>[4x]IEKKIVLRNGTEAFDSWEKPPLPVYTQFYFFNVTNPEEILRGETPRVEEVGPYTYRELRNKANIQFGDNGTTISAVSNKAYVFERDQSVGDPKIDLIRTLNIPVLTVIEWSQVHFLREIIEAMLKAYQQKLFVTHTVDELLWGYKDEILSLIHVFRPDISPYFGLFYEKNGTNDGDYVFLTGEDS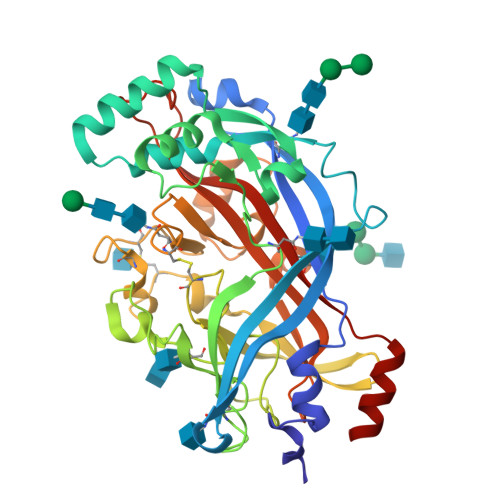YLNFTKIVEWNGKTSLDWWITDKCNMINGTDGDSFHPLITKDEVLYVFPSDFCRSVYITFSDYESVQGLPAFRYKVPAEILANTSDNAGFCIPEGNCLGSGVLNVSICKNGAPIIMSFPHFYQADERFVSAIEGMHPNQEDHETFVDINPLTGIILKAAKRFQINIYVKKLDDFVETGDIRTMVFPVMYLNESVHIDKETASRLKSMI> MTIQWFPGHMAKARREVTEKLKLIDIVYELVDARIPMSSRNPMIEDILKNKPRIMLLNKADKADAAVTQQWKEHFENQGIRSLSINSVNGQGLNQIVPASKEILQEKFDRMRAKGVKPRAIRALIIGIPNVGKSTLINRLAKKNIAKTGDRPG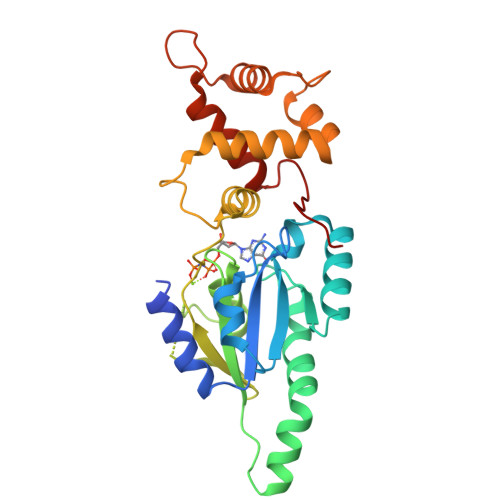ITTSQQWVKVGKELELLDTPGILWPKFEDELVGLRLAVTGAIKDSIINLQDVAVFGLRFLEEHYPERLKERYGLDEIPEDIAELFDAIGEKRGCLMSGGLINYDKTTEVIIRDIRTEKFGRLSFEQPTM2-chloro-L-phenylalanine | C9 H10 Cl N O2 | 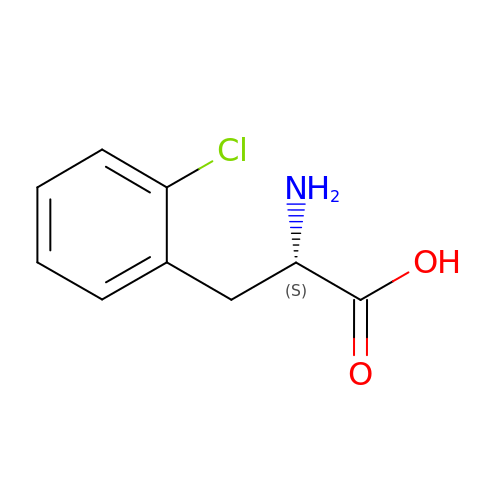CVZZNRXMDCOHBG-QMMMGPOBSA-N Metazoan mt-RNase P is a multi-enzyme assembly comprising the endonuclease PRORP and a tRNA methyltransferase (MTase) subcomplex composed of the MTase, TRMT10C, and the dehydrogenase, SDR5C1. We determined the structures of these four mt-tRNA maturation complexes using single-particle cryo-EM at a global resolution ranging from 2.7 to 3.2 Å, revealing snapshots of the four tRNA maturation steps, i.e. N1-methylation of purine 9, 5′-leader and 3′-trailer processing and 3′-CCA addition. The architecture of the maturation complexes is globally the same in all structures, i.e. TRMT10C asymmetrically straddles a tetramer of SDR5C1, while wrapping around the pre-tRNA. Our structures show that the TRMT10C/SDR5C1 complex can be a scaffold that presents mitochondrial pre-tRNAs as substrates for chemical modification, i.e. methylation, and nucleolytic cleavages at defined 5′ and 3′ sites and, finally 3′-CCA addition.

To investigate the dual specificity of TRMT10C, the methylation complexes were formed with pre-tRNAs containing either an A9 (pre-tRNAHis) or a G9 (pre-tRNAIle) and with S-adenosyl-L-homocysteine (SAH), the cofactor-product for methylation, bound in the TRMT10C active site. Methylation assays, using 3H-SAM as methyl donor, showed that the TRMT10C/SDR5C1 complex methylates both pre-tRNAIle and pre-tRNAHis-Ser. Single-particle cryo-EM data collection and processing yielded EM density maps at an overall resolution of 3.2 Å for the TRMT10C/SDR5C1/pre-tRNAIle complex, 2.7 Å for TRMT10C/SDR5C1/pre-tRNAHis-Ser/PRORP, 2.8 Å for TRMT10C/SDR5C1/pre-tRNAHis(0,Ser)/ELAC2 and 3.1 Å for TRMT10C/SDR5C1/tRNAIle /TRNT1. The density maps for the N-terminal domain (NTD) of TRMT10C were defined only for complexes where a maturation enzyme is bound on the pre-tRNA. In all the structures, the TRMT10C catalytic pocket contains SAH and the flipped-out substrate base: nucleotide A9 of pre-tRNAHis-Ser and nucleotide G9 of pre-tRNAIle. The flipped purine-9 is stacked against the conserved V313 and further stabilised in the TRMT10C active site by interaction with the same set of conserved residues, i.e. N222, Q226, D314 and N350. Q226 interacts with the N3 atom of A9 and with the N3 and NH2 group of G9, which are key for the selection of purines over pyrimidines. On the opposite side of purine-9, N348 and N350 interact with O6 and N7 of G9. The transferrable methyl group of SAM is located 3.0 Å from the N1 atom of A9 and 1.7 Å from G9 in the TRMT10C active site. Although no residue is in an appropriate position to allow the deprotonation of the N1 atom of G9, D314 appears to be the best catalytic candidate, and its mutation to alanine abolishes the TRMT10C N1-methylation activity.

>[4x]SVKGLVAVITGGASGLGLATAERLVGQGASAVLLDLPNSGGEAQAKKLGNNCVFAPADVTSEKDVQTALALAKGKFGRVDVAVNCAGIAVASKTYNLKKGQTHTLEDFQRVLDVNLMGTFNVIRLVAGEMGQNEPDQGGQRGVIINTASVAAFEGQVGQAAYSASKGGIVGMTLPIARDLAPIGIRVMTIAPGLFGTPLLTSLPEKVCNFLASQVPFPSRLGDPAEYAHLVQAIIENPFLNGEVIRLDGAIRMQP;> KNFLFLRLWDRNMDIAMGWKGAQAMQFGQPLVFDMAYENYMKRKELQNTVSQLLESEGWNRRNVDPFHIYFCNLKIDGALHRELVKRYQEKWDKLLLTSTEKSHVDLFPKDSIIYLTADSPNVMTTFRHDKVYVIGSFVDKSMQPGTSLAKAKRLNLATECLPLDKYLQWEIGNKNLTLDQMIRILLCLKNNGNWQEALQFVPKRKHTGFL> MPKTPHTKGPDETLSLLADPYRFISRQCQRLGANAFESRFLLKKTNCLKGAKAAEIFYDTTRFEREGAMPVAIQKTLLGQGGVQGLDGETHRHRKQMFMGLMTPERVRALAQLFEAEWRRAVPGWTRKGEIVFYDELHEPLTRAVCAWAGVPLPDDEAGNRAGELRALFDAAGSASPRHLWSRLARRRVDAWAKRIIEGIRA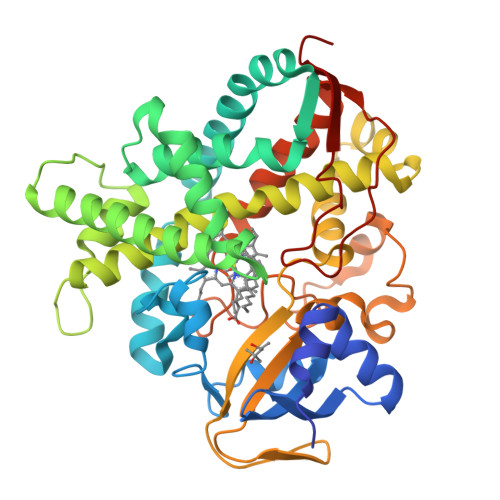GSIGSGSGTAAYAIAWHRDRHDDLLSPHVAAVELVNVLRPTVAIAVYITFVAHALQTCSGIRAALVQQPDYAELFVQEVRRFYPFFPAVVARASQDFEWEGMAFPEGRQVVLDLYGSNHDAATWADPQEFRPERFRAWDEDSFNFIPQGGGDHYLGHRCPGEWIVLAIMKVAAHLLVNAMRYDVPDQDLSIDFARLPALPKSGFVMRNVHIGG>[2x]GSSSGGSGHTPTTQATHADDHDLTTHNGTEEHDDGHDDGHDDLHAHAPKVIVFISGSCLFGAISRSLFKKLPIPYTVVLLILGAILGVVASNVPLVEEHTRDVAHMDPHVLLQIFLPVLIFESAFAMDVHTFMRSFSQVCILALFGLVVASVLTAVLAMNLFNYNWNFSEAMMFGAIMSATDPVAVVALLKDLGASKQLGTIIEGESLLNDGCAIVIFNVFMKMVFFPQLTSTVGQNVLYFLQVAVAGPLWGYAVAKVTVFFLSHIFNDALVEITITLAATYLTYYIGDIWLEVSGVLAVVVLGLIVNAEKTSISPEVEVFLHRFWEMLAYLANTLIFMMVGVVVTQKALVAVDKMDWFYLIILYLAITIIRGMVISLFSPILSRIGYGLTWRNAVIMTWGGLRGAVGLALALVVENLAGNDVIGSKFLFHTAGIVVLTLVINATTIQTLLRILGMSDISIPKRLAMAGAVRRIHEGQNRTLNMLKSDRFLADADWDIATAACEISDPYSALSDDENAPADELTLGERKSVCPGCKAMVPNEPSPREFADMMEEARLRMLKAEKISYWKQFEHG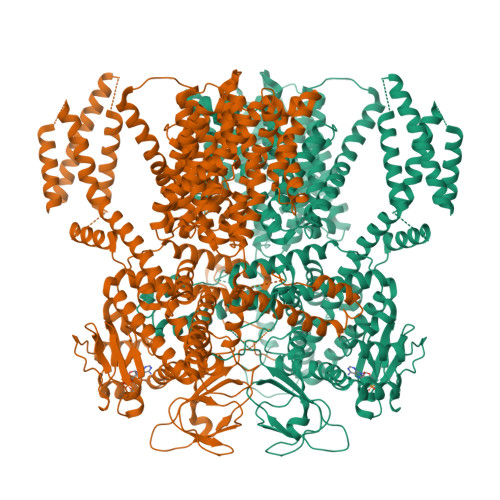MLAREALRLLVQHAEVAADEKDQFILVDDLKKSWQIKGIYPWLKRKLEDLISEKKIAAIPMPKYKLGKLMYKICHHMAFEVTINIAIVLNIVPIIMEFVVQDKMASVSTMAAPGSTVSSEPSSLQKIEDALRISNYVFFVIYAIEAIVKILGLGRHYIVSHWNKFDAFILVVALVDIIIAETLLKGSITINLSSIKVVKLFRLLRGLRMLRLTKALIPKLILVVNGKINNQLSLGYDVGKGYIIGEEEVGKIIDRMVDNKKILRELKHISETGRLQVVKELGLLQREHPGIAVSVKTRQAIRTILNHSRETIHELQGAGLLDEMEAHKLELTVEIKMKRLMNAPSSIPPPPPENLLKNVSWLAGDMKLIDFIKARASLLHFDYGEVIVREGDESDGLFLIVSGLVKLYGKSAFLDHDNPPVTAGSEENEVFEDYLTVGNVIGEMGVLTKKPRNATVTCETTVQVYFITAEDMNIAIDTFTLYPSLEYRLWRVVAIRIATPLIMEQMAFQGWTQEKVKLHLERGYLVDLAESHFQFNIDATLEDVILINGTAYNAHTREEIRSPCLISRTVHKLTFQYTATEEPRLFVVRNAEYNGPILDGRLDVDSKRSLISITEISSNMCL> QDPIKFTTGSATPASYNQFIDALRERLTGGLIYGIPVLRDPSTVEKPNQYVTVELSYSDTVSIQLGIDLTNAYVVAYRAGSESFFFRNAPASASTYLFTGTQQYSLPFDGNYDDLEKWAHQSRQRISLGLEALRQGIKFLRSGASDDEEIARTLIVIIQMVAEAARFRYVSKLVVISLSNRAAFQPDPSMLSLENTWEPLSRAVQHTVQDT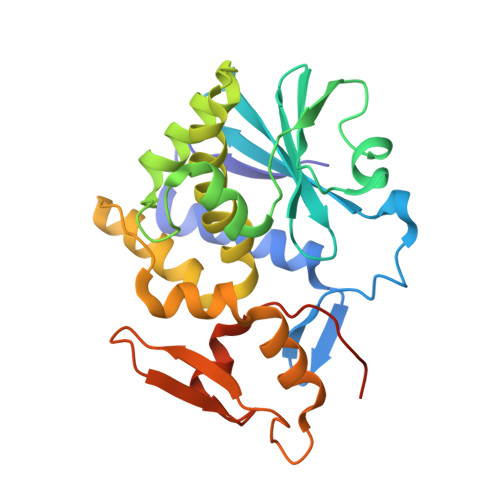FPQNVTLINVRQERVVVSSLSHPSVSALALMLFVCNPLNATQSPLLIRS4-{[6-(cyclohexylmethoxy)-7H-purin-2-yl]amino}-N,N-diethylbenzamide | C23 H30 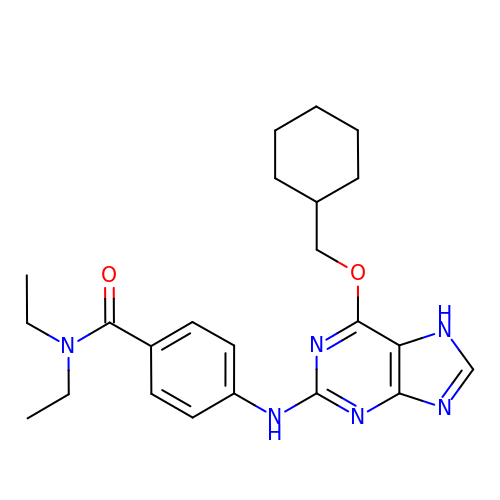N6 O2 | XHEQSRJCJTWWAH-UHFFFAOYSA-N> LTAPSIKSGTILHAWNWSFNTLKHNMKDIHDAGYTAIQTSPINQVKEGNQGDKSMSNWYWLYQPTSYQIGNRYLGTEQEFKEMCAAAEEYGIKVIVDAVINHTTFDYAAISNEVKSIPNWTHGNTQIKNWSDRWDVTQNSLLGLYDWNTQNTQVQSYLKRFLERALNDGADGFRFDAAKHIELPDDGSYGSQFWPNITNTSAEFQYGQILQDSASRDAAYANYMDVTASNYGHSIRSALKNRNLGVSNISHYASDVSADKLVTWVESHDTYANDDEESTWMSDDDIRLGWAVIASRSGSTPLFFSRPEGGGNGVRFPGKSQIGDRGSALFEDQAITAVNRFHNVMAGQPEELSNPNGNNQIFMNQRGSHGVVLANAGSSSVS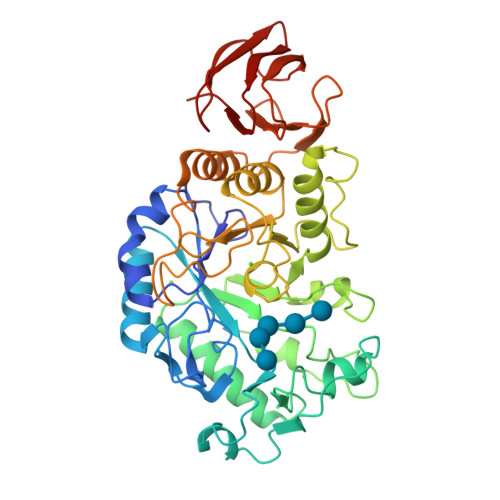INTATKLPDGRYDNKAGAGSFQVNDGKLTGTINARSVAVLYPD> MEDAKNIKKGPAPFYPLEDGTAGEQLHKAMKRYALVPGTIAFTDAHIEVNITYAEYFEMSVRLAEAMKRYGLNTNHRIVVCSENSLQFFMPVLGALFIGVAVAPANDIYNERELLNSMNISQPTVVFVSKKGLQKILNVQKKLPIIQKIIIMDSKTDYQGFQSMYTFVTSHLPPGFNEYDFVPESFDRDKTIALIMNSSGSTGLPKGVALPHRTACVRFSHARDPIFGNQIIPDTAILSVVPFHHGFGMFTTLGYLICGFRVVLMYRFEEELFLRSLQDYKIQSALLVPTLFSFFAKSTLIDKYDLSNLHEIASGGAPLSKEVGEAVAKRFHLPGIRQGYGLTETTSAILITPEGDDKPGAVGKVVPFFEAKVVDLDTGKTLGVNQRGELCVRGPMIMSG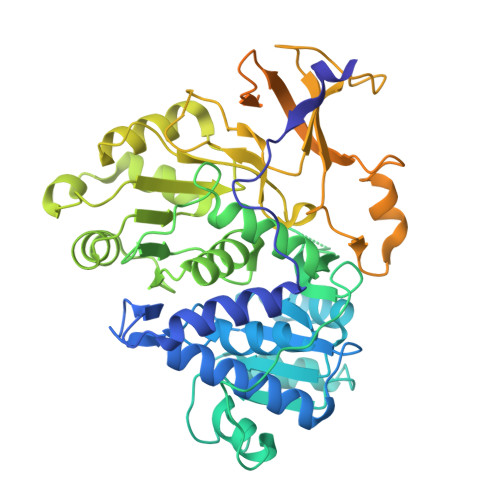YVNNPEATNALIDKDGWLHSGDIAYWDEDEHFFIVDRLKSLIKYKGYQVAPAELESILLQHPNIFDAGVAGLPDDDAGELPAAVVVLEHGKTMTEKEIVDYVASQVTTAKKLRGGVVFVDEVPKGLTGKLDARKIREILIKAKKGGKSKLV>[4x]MRKVKKLRLDKENTGSWRSFSLNSEGAERMATTG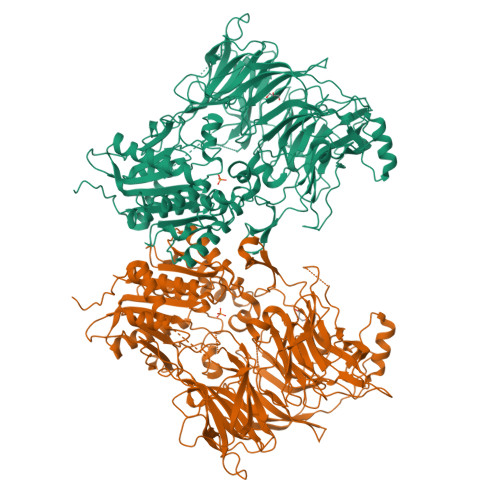TPTADRGDAAATDDPAARFQVQKHSWDGLRSIIHGSRKYSGLIVNKAPHDFQFVQKTDESGPHSHRLYYLGMPYGSRENSLLYSEIPKKVRKEALLLLSWKQMLDHFQATPHHGVYSREEELLRERKRLGVFGITSYDFHSESGLFLFQASNSLFHCRDGGKNGFMVSPMKPLEIKTQCSGPRMDPKICPADPAFFSFINNSDLWVANIETGEERRLTFCHQGLSNVLDDPKSAGVATFVIQEEFDRFTGYWWCPTASWEGSEGLKTLRILYEEVDESEVEVIHVPSPALEERKTDSYRYPRTGSKNPKIALKLAEFQTDSQGKIVSTQEKELVQPFSSLFPKVEYIARAGWTRDGKYAWAMFLDRPQQWLQLVLLPPALFIPSTENEEQRLASARAVPRNVQPYVVYEEVTNVWINVHDIFYPFPQSEGEDELCFLRANECKTGFCHLYKVTAVLKSQGYDWSEPFSPGEDEFKCPIKEEIALTSGEWEVLARHGSKIWVNEETKLVYFQGTKDTPLEHHLYVVSYEAAGEIVRLTTPGFSHSCSMSQNFDMFVSHYSSVSTPPCVHVYKLSGPDDDPLHKQPRFWASMMEAASCPPDYVPPEIFHFHTRSDVRLYGMIYKPHALQPGKKHPTVLFVYGGPQVQLVNNSFKGIKYLRLNTLASLGYAVVVIDGRGSCQRGLRFEGALKNQMGQVEIEDQVEGLQFVAEKYGFIDLSRVAIHGWSYGGFLSLMGLIHKPQVFKVAIAGAPVTVWMAYDTGYTERYMDVPENNQHGYEAGSVALHVEKLPNEPNRLLILHGFLDENVHFFHTNFLVSQLIRAGKPYQLQIYPNERHSIRCPESGEHYEVTLLHFLQEYLHHHHHH N-hydroxy-2-{[(4-methoxyphenyl)sulfonyl](2-{[(2R,3R,4S,5S,6R)-3,4,5-trihydroxy-6-(hydroxymethyl)tetrahydro-2H-pyran-2-yl]oxy}ethyl)amino}acetamide 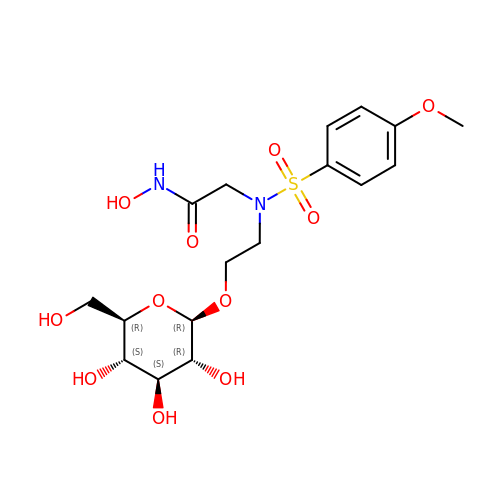| C17 H26 N2 O11 S | RBZQWZODGBMNHX-USACIQFYSA-N>[8x]MTIKALRTPEERFSVLPAFPYQPNYVDDLGGYESLRMAYIDEGDKDSEYTFLCLHGEPTWSYLYRKMIPVFTDAGHRV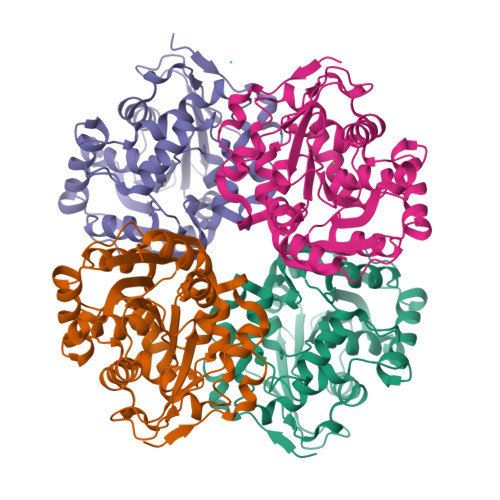VAPDLFGFGRSDKPIEDSVYNFEFHRNSLIQLIEHLDLKNIVLVCQDWGGGLGLTIPMDMQDRFKKLIVMNTTISNGEPLAEAAVQWMAFNETISELPVAGLVACDAGAAVNVMDALAYDAPFPNKNYKVGVKRFPQMIPTNADDDAVKYGLRAIEFWSNEWSGESFMAIGMKDAVLGEAAMMQLKTVIKGCPEPMKIEEAGHFVQEYGVEVAEQALASFTMIHHHHHH> MTATQGKCPVMHGGATTVNISTAEWWPKALNLDILSQHDRKTNPMGPDFNYQEEVKKLDVAALKQDLQALMTDSQDWFPADWGHYGGLMIRLTWHAAGTYRIADGRGGAGTGNQRFAPLNSWPDNTNLDKARRLLWPIKQKYGNKLSWADLIAYAGTIAYESMGLKTFGFAFGREDIWHPEKDIYWGPEKEWVPPSTNPNSRYTGDRELENPLAAVTMGLIYVNPEGVDGNPDPLKTAHDVRVTFARMAMNDEETVALTAGGHTVGKCHGNGNAALLGPEPEGADVEDQGLGWINKTQSGIGRNAVTSGLEGAWTPHPTQWDNGYFRMLLNYDWELKKSPAGAWQWEPINPREEDLPVDVEDPSIRRNLVMTDADMAMKMDPEYRKISERFYQDPAYFADVFARAWFKLTHRDMGPKARYIGPDV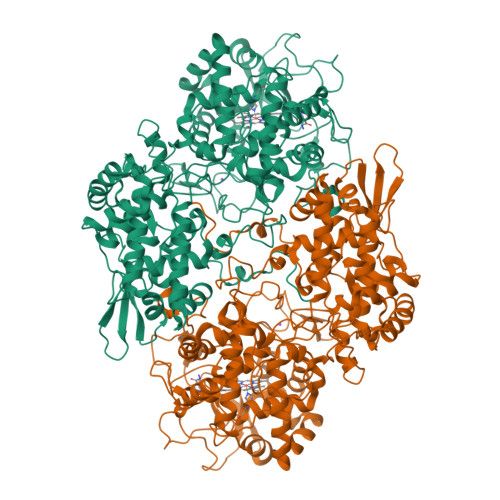PQEDLIWQDPIPAGNRNYDVQAVKDRIAASGLSISELVSTAWDSARTYRNSDKRGGANGARIRLAPQKDWEGNEPDRLAKVLAVLEGIAAATGASVADVIVLAGNVGVEQAARAAGVEIVLPFAPGRGDATAEQTDTESFAVLEPIHDGYRNWLKQDYAATPEELLLDRTQLLGLTAPEMTVLIGGLRVLGTNHGGTKHGVFTDREGVLTNDFFVNLTDMNYLWKPAGKNLYEICDRKTNQVKWTATRVDLVFGSNSILRAYSELYAQDDNKEKFVRDFVAAWTKVMNADRFDLD>[2x]SHMLRPVETPTREIKKLDGLWAFSLDRENCGIDQRWWESALQESRAIAVPGSFNDQFADADIRNYAGNVWYQREVFIPKGWAGQRIVLRFDAVTHYGKVWVNNQEVMEHQGGYTPFEADVTPYVIAGKSVRITVCVNNELNWQTIPPGMVITDENGKKKQSYFHDFFNYAGIHRSVMLYTTPNTWVDDITVVTHVAQDCNHASVDWQVVANGDVSVELRDADQQVVATGQGTSGTLQVVNPHLWQPGEGYLYELCVTAKSQTECDIYPLRVGIRSVAVKGEQFLINHKPFYFTGFGRHEDADLRGKGFDNVLMVHDHALMDWIGANSYRTSHYPYAEEMLDWADEHGIVVIDETAAVGFNLSLGIGFEAGNKPKELYSEEAVNGETQQAHLQAIKELIARDKNHPSVVMWSIANEPDTRPQGAREYFAPLAEATRKLDPTRPITCVNVMFCDAHTDTISDLFDVLCLNRYYGWYV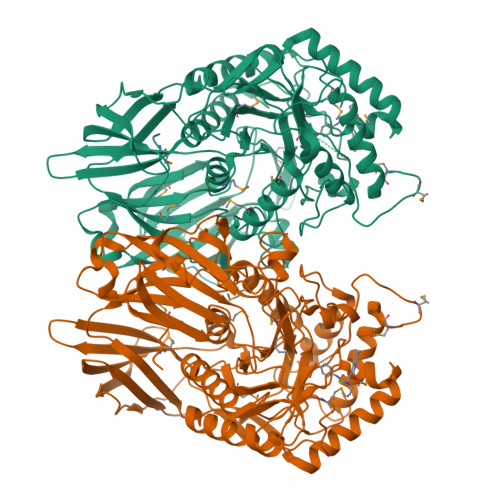QSGDLETAEKVLEKELLAWQEKLHQPIIITEYGVDTLAGLHSMYTDMWSEEYQCAWLDMYHRVFDRVSAVVGEQVWNFADFATSQGILRVGGNKKGIFTRDRKPKSAAFLLQKRWTGMNFGEKPQQGGKQ2-methoxypropanedioic 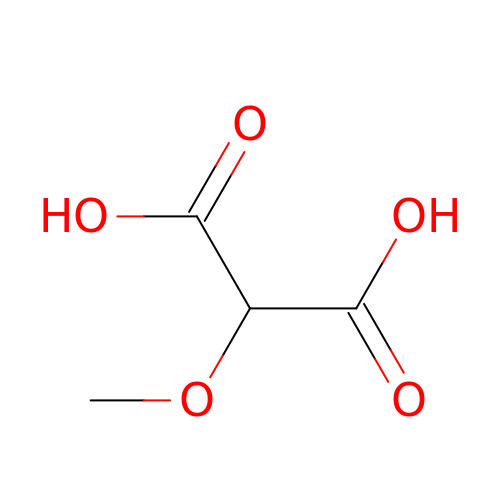acid | C4 H6 O5 | VLDSMCHWNWDAKQ-UHFFFAOYSA-N> MIIPALDLIDGTVVRVVRLHQGDYARQRDYGNDPLPRLQDYAAQGAGVLHLVDLTGAKDPAKRQIPLIKTLVAGVNVPVQVGGGVR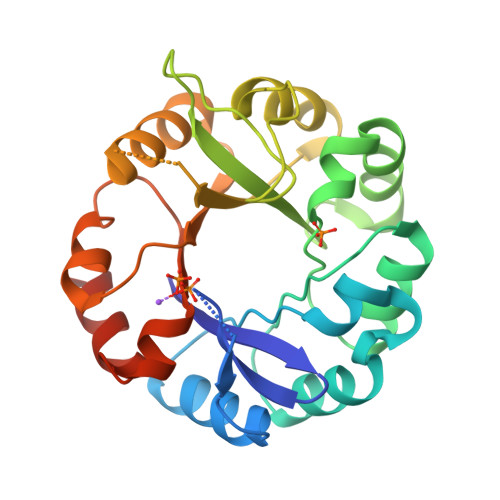TEEDVAALLKAGVARVVIGSTAVKSPDVVKGWFERFGAQALVLALDVRIDEHGTKQVAVSGWQENSGVSLEQLVETYLPVGLKHVLCTDISRDGTLAGSNVSLYEEVCARYPQIAFQSSGGIGDIDDIAALRGTGVRGVIVGRALLEGKFTVKEAIQCWQNVKGHHHHHH>[2x]MRGSHHHHHHGLVPRGSMIRTMLQGKLHRVKVTHADLH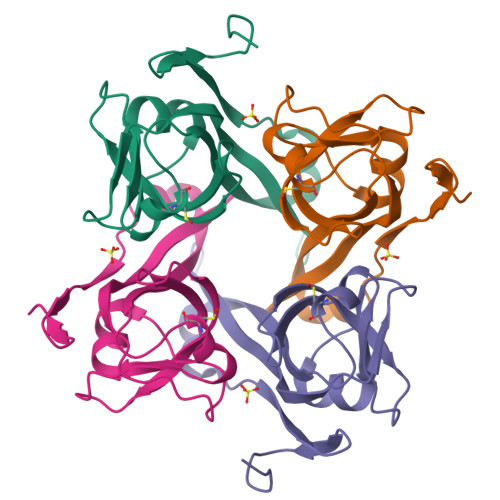YESSCAIDQDFLDAAGILENEAIDIWNVTNGKRFSTYAIAAERGSRIISVNGAAAHCASVGDIVIIASFVTMPDEEARTWRPNVAYFEGDNEMKRTAKAIPVQVA>GSMDIALHGGAWHESLGKLLEALDRPFFWRILAQTLGQFAPVDNWAALIFSDSSPLILSFMEEEREEVEPDPLISRYITGLYLQDPFYQVSRNCRRGG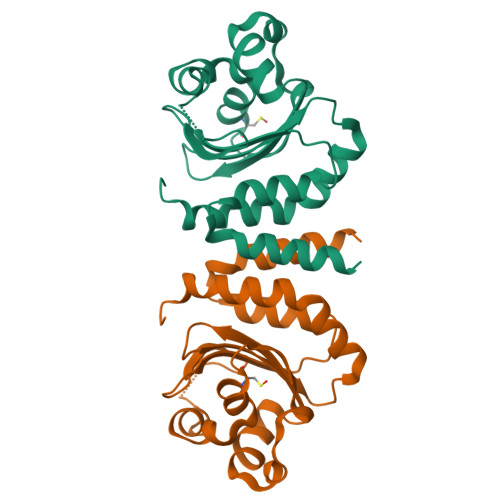LFHLADIVSEDFETTEYYNTYFAHYVVTDEVQYNVPLDGERTLCLSLGSESRFGAEQIALFELLRPWVIALMKKRIHFEDAVREEAKPIAAAEVEVQ[2x]> MAANKPKGQNSLALHKVIMVGSGGVGKSALTLQFMYDEFVEDYEPTKADSYRKKVVLDGEEVQIDILDTAGQEDYAAIRDNYFRSGEGFLCVFSITEMESFAATADFREQILRVKEDENVPFLLVGNKSDLEDKRQVSVEEAKNRAEQWNVNYVETSAKT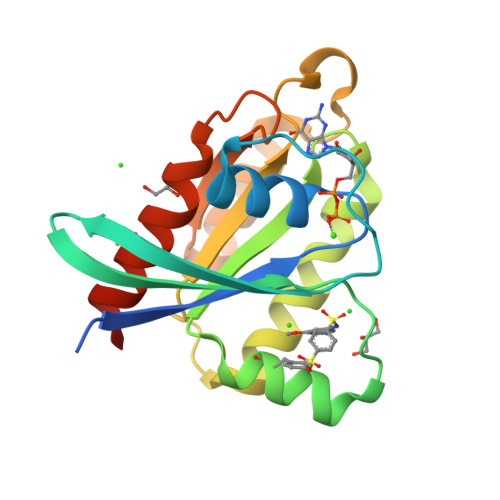RANVDKVFFDLMREIRARLEHHHHHH> GAMDAAVEPEERHLSKMQQNGYEN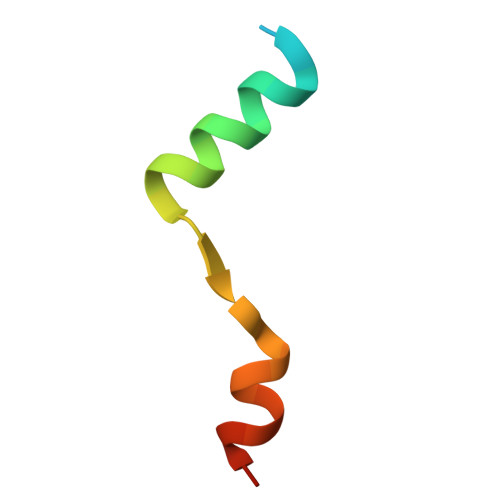PTYKFFEQMQN>MIFDKEDYKAFDPELWNAIDAEAERQQNNIELIASENVVSKAVMAAQGTLLTNKSAEGYPGKRYYGGTAVIDVVETLAIERAKKLFGAKFANVQPHSGSQANAAVYMSLIQPGDTVMGMDLSAGGHLTHGAPVSFSGKTYNFVSYNVDKESELLDYDAILAQAKEVRPKLIVAGASAYSRIIDFAKFREIADAVGAYLMVDMAHIAGLVASGHHPSPVPYAHVTTTTTHKTLRGPRGGLILTDDEDIAKKLNSAVFPGLQGGPLEHVIAAK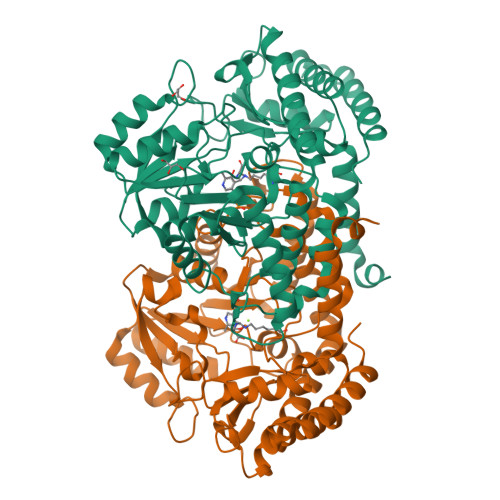AVALKEALDPAFKEYGENVIKNAAAMADVFNQHPDFRVISGGTNNHLFLVDVTKVVENGKVAQNVLEEVNITLNKNSIPYEQLSPFKTSGIRVGSPAITSRGMGEAESRQIAEWMVEALENHDKPEVLERIRGDVKVLTDAFPLY[2x]> MAKRRGRGAATFAALGFGAAAGIAFGTYVLAPNLPENIDPNAPTSAELVEAETLAEVNAVQADQADSIIDHIVEDVVAGTLTDRPVLVMRTADAEESDV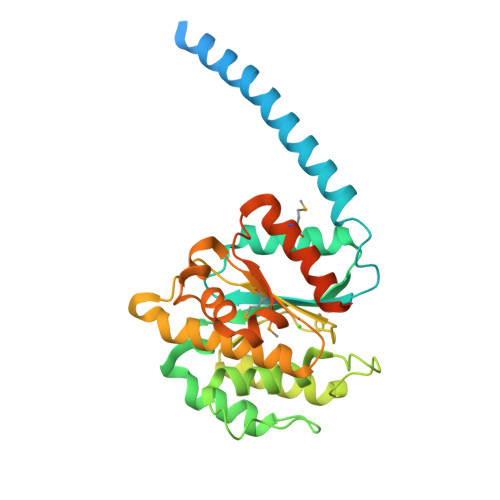ADVSWLLQQAGAINAGSITLEENFFSQDGADQLKSIVANTLPAGAQLSETQLDPGTHAGEALGAALLLNPETGEPLASTAERGLLLNVLRDNGYISYEDGTILPGQVIVMITGDSDGSGDGAFAAETQSLFARALDAQGSGVVVAGRIHTAADTGVIGRLRANPDAAENVSTIDSVNRTWGKMATVLSVREELAGRSGAFGSAASADAASPSLDGTAAAPAQ> MAKKTSSKGKLPPGPRPLPLLGNLLQMDRRGLLKSFLRFREKYGDVFTVHLGPRPVVMLCGVEAIREALVDKAEAFSGRGKIAMVDPFFRGYGVIFANGNRWKVLRRFSVTTMRDFGMGKRSVEERIQEEAQCLIEELRKSKGALMDPTFLFQSITANIICSIVFGKRFHYQDQEFLKMLNLFYQTFSLISSVFGQLFELFSGFLKHFPGAHRQVYKNLQEINAWIGHSVEKHRETLDPSAPRDLIDTYLLHMEKEKSNAHSEFSHQNLNLNTLSLFFAGTETTSTTLRYGFLLMLKYPHVAERVYREIEQVIGPHRPPELHDRAKMPYTEAVIYEIQRFSDLLPMGVPHIVTQHTSFRGYIIPKDTEV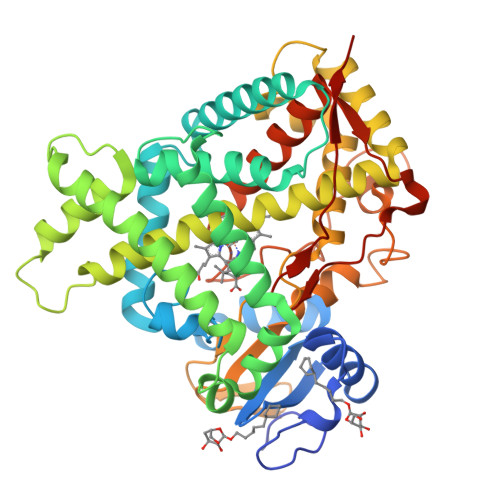FLILSTALHDPHYFEKPDAFNPDHFLDANGALKKTEAFIPFSLGKRICLGEGIARAELFLFFTTILQNFSMASPVAPEDIDLTPQECGVGKIPPTYQIRFLPRHHHH> SHMLRSSLLPFSYLYEKIINFRNTLYDKGFLKIKKLPVPVISV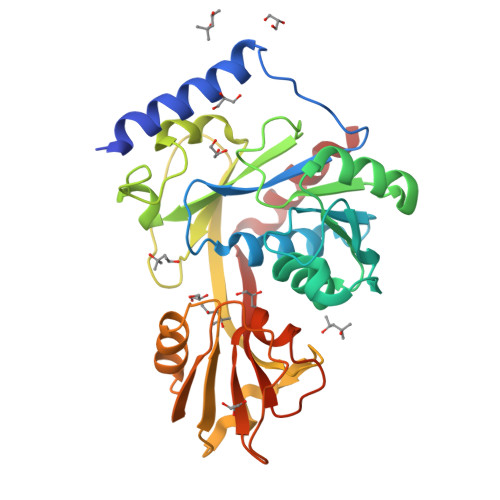GNLSVGGSGKTSFVMYLADLLKDKRVCILSRGYKRKSKGTLIVSEYGNLKVSWEEAGDEPYLMAKLLPHVSVVASEDRYKGGLLALEKLSPEVFILDDGFQHRKLHRDLNILLLKKKDLKDRLLPAGNLREPLKEIRRADALVLTYQEVEPFEFFTGKPTFKMFREFCCLLNSDFEEVPFDILKEREVIAFSGLGDNGQFRKVLKNLGIKVKEFMSFPDHYDYSDFTPEEGEIYLTTPKDLIKLQGYENVFALNFKVKLEREEKLKKLIYRIFY>MKKRLTESQFQEAIQGLEVGQQTIEIARGVLVDGKPQATFATSLGLTRGAVSQAVHRVWAAFEDKNLPEGYARVTAVLPEHQAYIV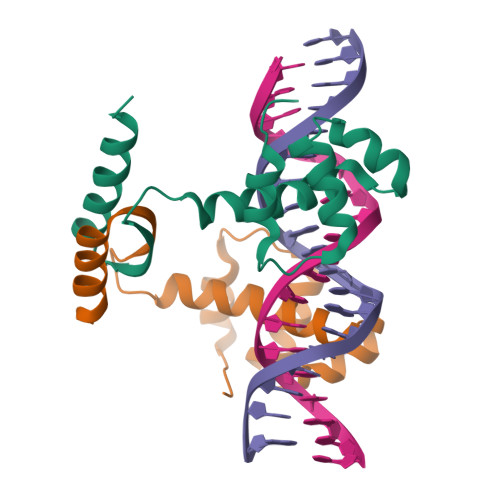RKWEADAKKKQ[2x]2-{[(2E)-4-chlorobut-2-enoyl]amino}-2-deoxy-beta-D-glucopyranose 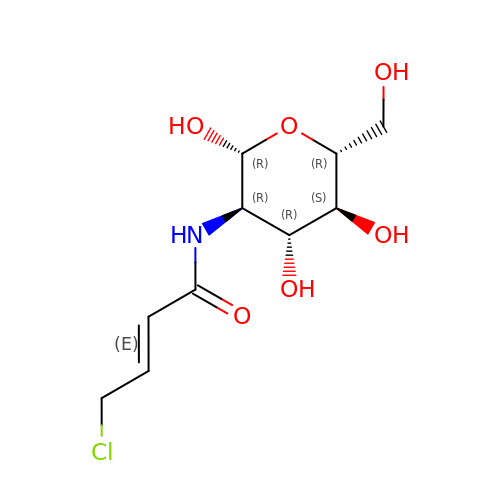| C10 H16 Cl N O6 | LKECTNVLFDGIBK-KKRTVAFTSA-N>[2x]MSLQLLRNTRIFVSTVKTGHNKTNTQEILVQDDISWGQDSNSTDITVNEAGPRPTRGSKRFNDSLNAAEWSFSTYILPYKDKNTSKQIVPDYMLWHALSSGRAINLEGTTGAHNNATNFMVNFKDNSYHELAMLHIYILTDKTWSYIDSCQINQAEVNVDIEDIGRVTWSGNGNQLIPLDEQPFDPDQIGIDDETYMTIQGSYIKNKLTILKIKDMDTNKSYDIPITGGTFTINNNITYLTPNVMSRVTIPIGSFTGAFELTGSLTAYLNDKSLGSMELYKDLIKTLKVVNRFEIALVLGGEYDDERPAAILVAKQAHVNIPTIETDDVLGTSVEFKAIPSDLDAGDEGYLGFSSKYTRTTINNLIVNGDGATDAVTAITVKSAGNVTTLNRSATLQMSVEVTPSSARNKEVTWAITAGDAATINATGLLRADASKTGAVTVEATAKDGSGVKGTKVITVTAGGENLYFQGHHHHHH

Phage T5 is a Siphoviridae infecting the Gram-negative host Escherichia coli. In T5, the tail tube is formed by the stack of 40 trimers of the TTP pb616 around the tape measure protein (TMP). Here, we determined the structure of pb6, and show that it results in the duplication/fusion of the hexamerisation domain common to all other tubes. Thus, T5 TTP is not an outlier in the family of TTPs, as it contains the same hexamerisation domain as other phages, T6SS and pyocin tube proteins, but results from a duplication/fusion: the unusual threefold symmetry of the tube is in fact pseudo-hexameric.

We have determined the pb6 monomer structure at 2.2 Å resolution. At first sight, the structure can be divided into two domains encompassing 374 and 85 residues. The C-terminal domain (residues 375–462) possesses an immunoglobulin-like (Ig-like) fold of the Big-2 family, confirming a previous sequence analysis. In λ, however, its absence has an influence on burst size and temperature sensitivity of the phage particle. For pb6, formation of tubes occurs even when this domain is absent (see below), and some T5-like TTP lack it. The common core shared by both subdomains consists of a β-sandwich flanked by an α-helix, and a long loop. This loop is not resolved in subdomain 1 (loop β3–β4), whereas it is stabilised by crystal contacts in subdomain 2 (loop β13–β14). However, both subdomains display high structural homology with TTPs of other sipho- and myophages, distal tail proteins of siphophages, T6SS tube proteins, the tube protein of R-pyocin, baseplate hub proteins from myophages and spike proteins from T6SS. The X-ray structure of the pb6 monomer fits remarkably well in the tube density (Chimera correlation 0.89 using a pb6 map simulated from atoms at a resolution of 6 Å, 879/6657 atoms being outside the contour), except for the N terminus, the long β13–β14 loop, loop β17–β18 and helix α5, all positioned at interfaces between monomers. Interestingly, these elements have a high temperature factor—i.e., are more flexible—in the crystal structure, and we could model them and loop β3–β4 in the unassigned EM densities observed in their vicinity, leading to a complete pseudo-atomic model of the T5 tail tube. In the tube assembly, a monomer is connected to six neighbouring subunits, making this structure very stable (pb6 tube melting temperature = 83 °C vs. 50 °C for pb6 monomer; note that it is 90 °C for purified tails).> ESKKRQWALEDFEIGRPLGKGKFGNVYLAREKQSKFILALKVLFKAQLEKAGVEHQLRREVEIQS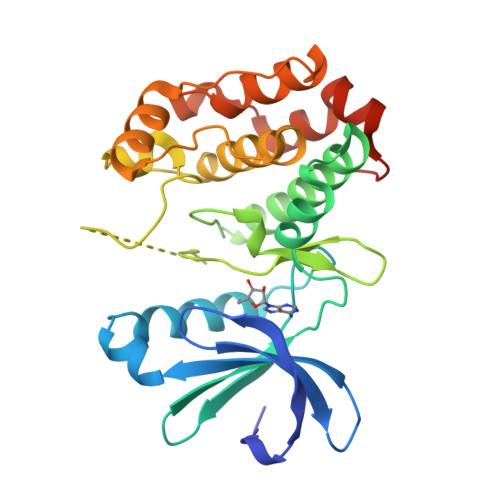HLRHPNILRLYGYFHDATRVYLILEYAPLGTVYRELQKLSKFDEQRTATYITELANALSYCHSKRVIRRDIKPENLLLGSAGELKIADFGWSVHAPSSRRTTLCGTLDYLPPEMIEGRMHDEKVDLWSLGVLCYEFLVGKPPFEANTYQETYKRISRVEFTFPDFVTEGARDLISRLLKHNPSQRPMLREVLEHPWITANSSKPSNCQNKESASKQS> MSSNTFTEEGRLLQTEYAIKNVSKGGTIIGLVCKDGVILLGINKTELLDEREKIYKINPKVYVSVSGLFGDAMLLKKYGQVKAQDFLYEFDYDCDIDRICNFISEKKQLFTQYNSTRPFGFSFIYAGMKNNKFKLCSTDPSGTINEWKGVCFGENED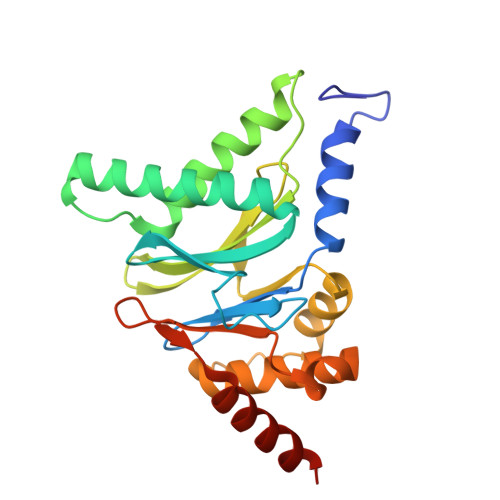AINNGLRNDFPDEEMDMERGLFEIFKILSKVTECSAKDHKKYEILYFKNEESRFLEFEEIENILLRIEEEKNKK>MGITLGEVFPNFEADSTIGKLKFHDWLGNSWGVLFSHPRDFTPVSTTELGRVIQLEGDFKKRGVKLIALSCDNVADHKEWSEDVKCLSGVKGDMPYPIIADETRELAVKLGMVDPDERTSTGMPLTCRAVFIIGPDKKLKLSILYPATTGRNFSEILRVIDSLQLTAQKKVATPADWQPGDRCMVVPGVSAEEAKTLFPNMEVKAVPSGKGYLRYTPQPK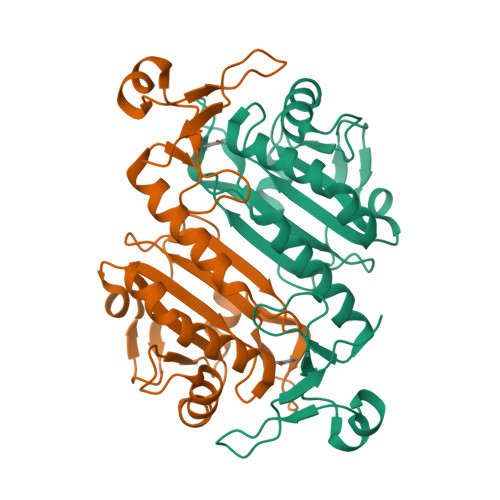SMGGSRSHHHHHH[4x]> XSLSDKDKAAVRALWSKIGKSSDAIGNDALSRMIVVYPQTKIYFSHWPDVTPGSPNIKAHGKKVMGGIALAVSKIDDLKTGLMELSEQHAYKLRVDPSNFKILNHCILVVISTMFPKEFTPEAHVSLDKFLSG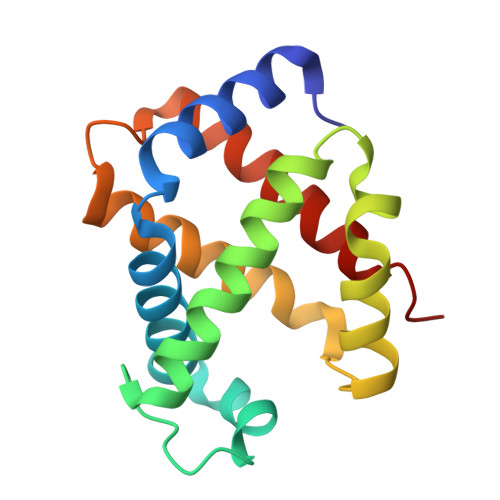VALALAERYR> SENLKDEILEKYIPKTKKTRSGHIVIKTEETPNPEIVANTRTVPGIITARGCAYAGCKGVVMGPIKDMVHITHGPIGCSFYTWGGRRFKSKPENGTGLNFNEYVFSTDMQESDIVFGGVNKLKDAIHEAYEMFHPAAIGVYATCPVGLIGDDILAVAATASKEIGIPVHAFSCEGYKGVSQSAGHHIANNTVMTDIIGKGNKEQKKYSINVLGEYNIGGDAWEMDRVLEKIGYHVNATLTGDATYEKVQNADKADLNLVQCHRSINYIAEMMETKYGIPWIKCNFIGVDGIVETLRDMAKCFDDPELTKRTEEVIAEEIAAIQDDLDYFKEKLQGKTACLYVGGSRSHTYMNMLKSFGVDSLVAGFEFAHRDDYEGREVIPTIKIDADSKNIPEITVTPDEQKYRVVIPEDKVEELKKAGVPLSSYGGMMKEMHDGTILIDDMNHHDMEVVLEKLKPDMFFAGIKEKFVIQKGGVLSKQLHSYDYNGPYAGFRGVVNFGHELVNG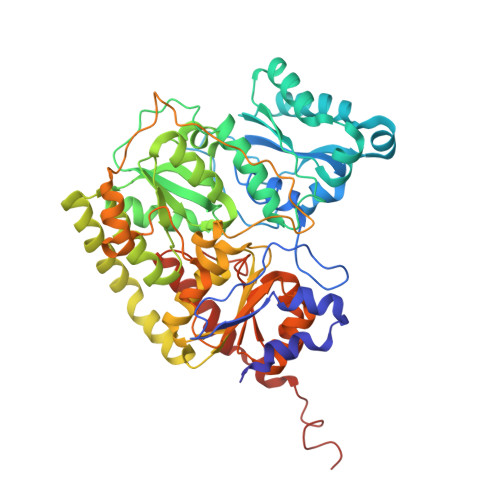IYTPAWKMITPPWKKASSESKVVVGGEA> LLTPPPPPL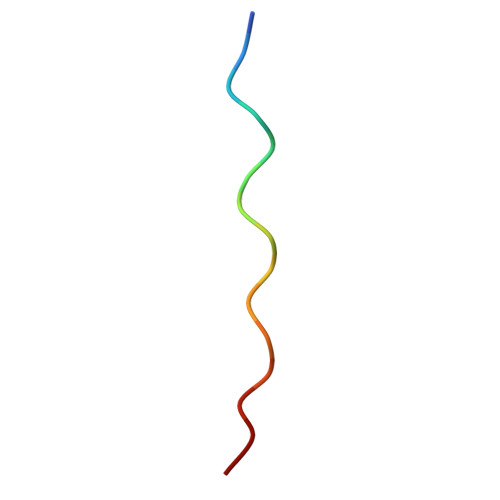FPPPFF>[2x]GPSGGGADVNKGPWAMALTPMEFARKYN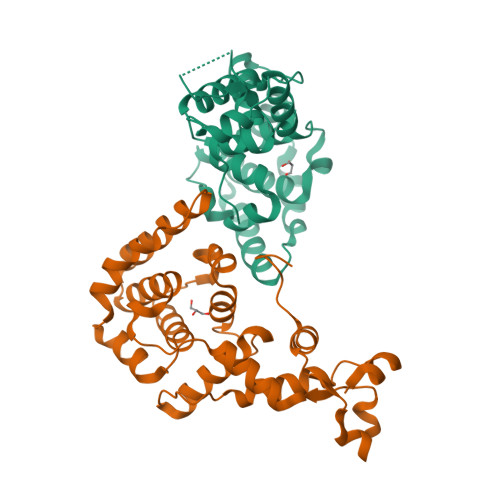LLRKDDALLDNPVPGEEMTAGIRRGDAKRVFTMQLGPYWDGFERCSPQAYALSAVFMARMNRDRDAANNILKVLDKTFVDGKPDFSVARPVMKKYQNSELVQEVVAKHAYVLTVIASLLEAAREDGVVPSSEFLWLKPVDRRLWYMLNCVGRQTPYSEVAGPFAHWKAEKEMGRRSLVPMIDEAIRALEIAVKEVRLTPRQMEELEP> MSPENPWLWAVLVLLLALSAFFSASETAITTLYPWK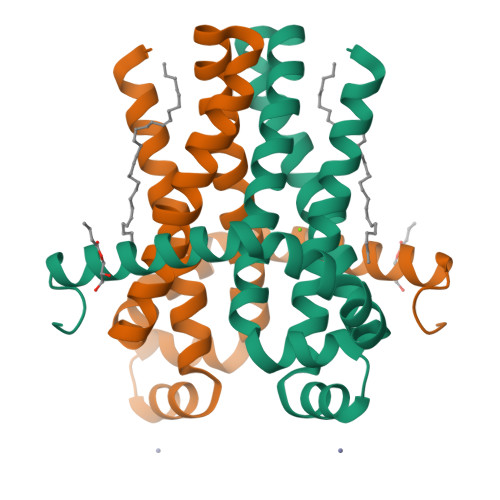LKELAESKNGPFRLLAEDITRFLTTILVGNNLVNIAATALVTELATQAFGSAGVGVATGAMTFLILFFGEITPKSLAVHHAEAIARLAAWPIYGLSVLFYPVGRFFSLVSGGLLRLLGLEPRLESSGLEVLFQ>[2x]MLEIKRYKNRVASRKCRAKFKQLLQHYREVAAAKS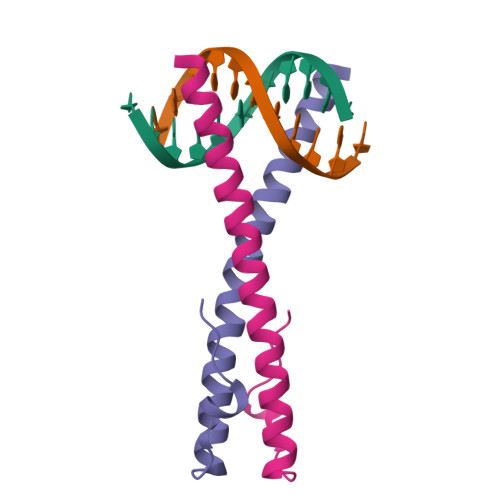SENDRLRLLLKQMCPSLDVDSIIPRTPD>SKGSAVTTPQNNDEEYLTPVTVGKSTLHLDFDTGSADLWVFSDELPSSEQTGHDLYTPSSSATKLSGYSWDISYGDGSSASGDVYRD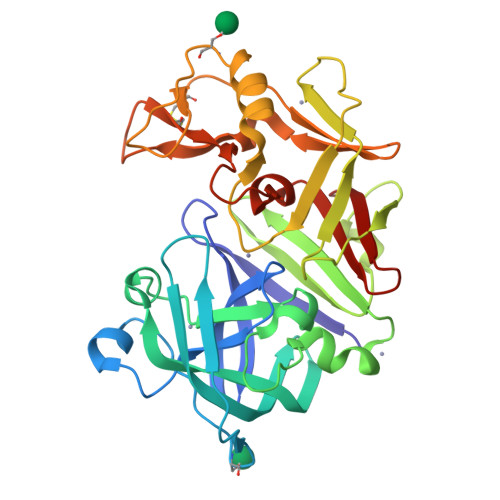TVTVGGVTTNKQAVEAASKISSEFVQDTANDGLLGLAFSSINTVQPKAQTTFFDTVKSQLDSPLFAVQLKHDAPGVYDFGYIDDSKYTGSITYTDADSSQGYWGFSTDGYSIGDGSSSSSGFSAIADTGTTLILLDDEIVSAYYEQVSGAQESYEAGGYVFSCSTDLPDFTVVIGDYKAVVPGKYINYAPVSTGSSTCYGGIQSNSGLGLSILGDVFLKSQYVVFNSEGPKLGFAAQA[2x]>MKAPVRVAVTGAAGQIGYSLLFRIAAGEMLGKDQPVILQLLEIPQAMKALEGVVMELEDCAFPLLAGLEATDDPKVAFKDADYALLVGAAPRKAGMERRDLLQVNGKIFTEQGRALAEVAKKDVKVLVVGNPANTNALIAYKNAPGLNPRNFTAMTRLDHNRAKAQLAKKTGTGVDRIRRMTVWGNHSSTMFPDLFHAEVDGRPALELVDMEWYEKVFIPTVAQRGAAIIQARGASSAASAANAAIEHIRDWALGTPEGDWVSMAVPSQGEYGIPEGIVYSFPVTAKDGAYRVVEGLEINEFARKRMEITAQELLDEMEQVKALGLIRKLAAALEHHHHHH[4x]

Malate dehydrogenase (MDH, EC 1.1.1.37) catalyzes a dehydrogenation reaction from malic acid to generate oxaloacetic acid, which is accompanied by reduced NAD generating NADH. MDH from T. thermophilus (TtMDH) is more similar in amino acid sequence to NADP-dependent chloroplastic MDH than NAD-dependent bacterial and mitochondrial MDHs. The molecular mass of TtMDH in solution determined by analytical gel filtration chromatography was about 61 kDa, so TtMDH is a homodimeric enzyme like most MDHs. Similar to other MDHs, a protomer of TtMDH has the N-terminal NAD binding domain and C-terminal catalytic domain and consists of 12 helices and 11 β-strands.

To gain further insight into the co-substrate recognition and activity relationship for TtMDH, we attempted to soak the apo-form crystal with NAD. In addition, we found a mass of electron density in co-substrate binding site of TtMDH that could be modeled as NAD. Unlike the apo form of TtMDH, crystal structure of NAD-bound TtMDH belongs to the P212121 space group with four molecules in an asymmetric unit; however, a homodimer should be formed with identical subunits in the crystal lattice. Nevertheless, electron densities for residues 91–100 were relatively weak and poorly defined. They correspond to the mobile loop covering the catalytic site, which is disordered as in the 3D structures of most other MDHs. NAD binds to TtMDH in the same extended conformation seen for other members of this enzyme family. The adenine ring binds in a hydrophobic crevice defined by Leu41, Ile43, Ile108, Thr10, Gly11, Gly88, and the backbone of Gly88 and Ala89. Residue 42 of TtMDH is a glutamate, which hydrogen-bonds to the adenine ribose instead of the otherwise conserved aspartate in other MDHs. The NAD pyrophosphate is hydrogen-bonded to the backbone of residue 15 and 16, but nicotinamide ribose is hydrogen-bonded to the side-chain of residue Asn131 through 2′-hydroxyl. However, the increasing B-factor value, slight movement of the binding loop and few structural elements around the NAD binding site indicate that conformational change is significant for TtMDH activity.> MVRIIVKNVSKV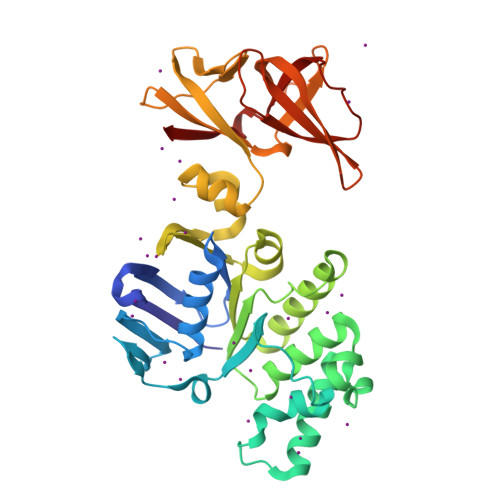FKKGKVVALDNVNINIENGERFGILGPSGAGKTTFMRIIAGLDVPSTGELYFDDRLVASNGKLIVPPEDRKIGMVFQTWALYPNLTAFENIAFPLTNMKMSKEEIRKRVEEVAKILDIHHVLNHFPRELSGGQQQRVALARALVKDPSLLLLDEPFSNLDARMRDSARALVKEVQSRLGVTLLVVSHDPADIFAIADRVGVLVKGKLVQVGKPEDLYDNPVSIQVASLIGEINELEGKVTNEGVVIGSLRFPVSVSSDRAIIGIRPEDVKLSKDVIKDDSWILVGKGKVKVIGYQGGLFRITITPLDSEEEIFTYSDHPIHSGEEVLVYVRKDKIKVFEKN>[2x]GPLGSDQYIVVNGAPVIPSAKVPVLKKALTSLFSK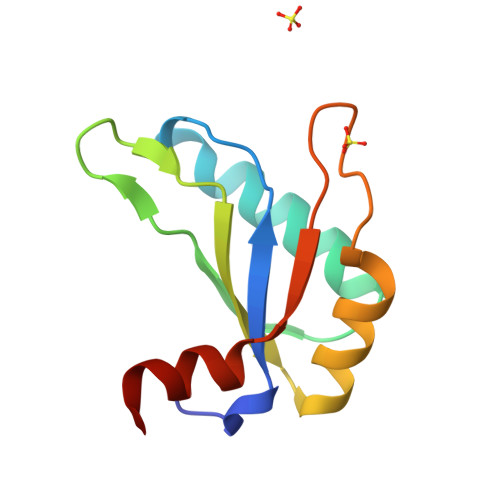AGKVVNMEFPIDEATGKTKGFLFVECGSMNDAKKIIKSFHGKRLDLKHRLFLYTMKDVERYNSDD> GSHMGSPNSPLKDSLRPKLSEEQQHIIAILLDAHHKTYDPTYADFRDFRPPVRMDGSTGSVTLDLSPLSMLPHLADLVSYSIQKVIGFAKMIPGFRDLTSDDQIVLLKSSAIEVI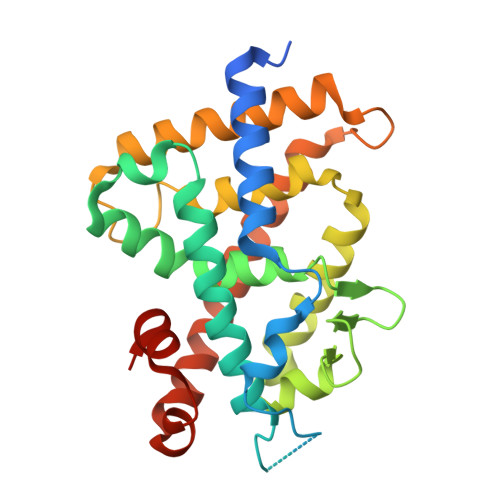MLRSNQSFTMDDMSWDCGSQDYKYDVTDVSKAGHTLELIEPLIKFQVGLKKLNLHEEEHVLLMAICIVSPDRPGVQDAKLVEAIQDRLSNTLQTYIRCRHPPPGSHQLYAKMIQKLADLRSLNEEHSKQYRSLSFQPENSMKLTPLVLEVFGNEIS> GAQVSTQKTGAHETGLSASGNSI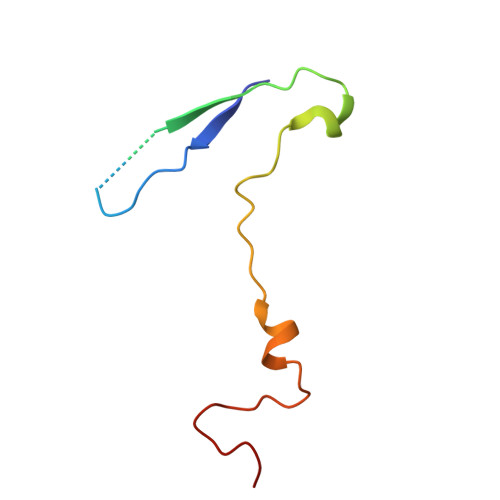IHYTNVNYYKDAASNSANRQDFTQDPGKFTEPVKDIMIKSMPALN>MGSMENPLFDYYRNRQAPLQWRGALGALAQSLTNHFSPEQLRTLLREAGQHFASQHPVQAAETVQSMQD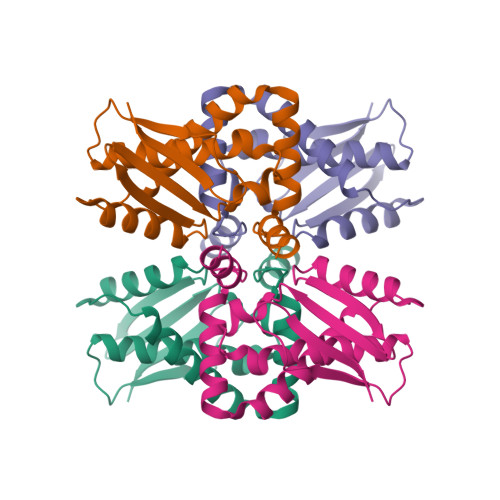AMNGVWTTQDWGWVDIHDLDSFLTLTHYAAPLESAFGAQNLAWSAAFLEGVYEQWFRQLGASDALHVRQSEESDVRKAIVLRLGR[4x]>PYVEIIEQPKQRGMRFRYKCEGRSAGSIPGERSTDTTKTHPTIKINGYTGPGTVRISLVTKDPPHRPHPHELVGKDCRDGYYEADLCPDRSIHSFQNLGIQCVKKRDLEQAISQRIQTNNNPFHVPIEEQRGDYDLNA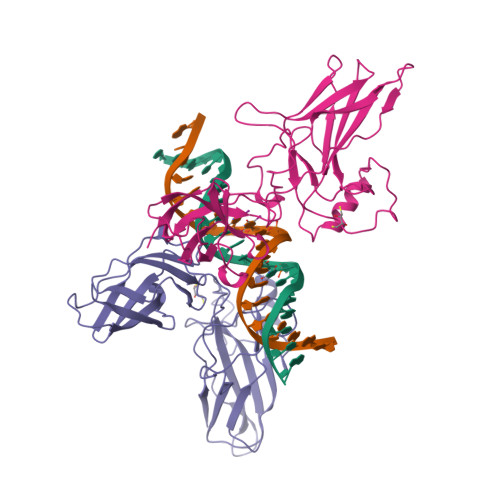VRLCFQVTVRDPAGRPLLLTPVLSHPIFDNRAPNTAELKICRVNRNSGSCLGGDEIFLLCDKVQKEDIEVYFTGPGWEARGSFSQADVHRQVAIVFRTPPYADPSLQAPVRVSMQLRRPSDRELSEPMEFQYLPD[2x]>STNLVAEPFAKLEQDFGGSIGVYAMDTGSGATVSYRAEERFPLCSSFKGFLAAAVLARSQQQAGLLDTPIRYGKNALVPWSPISEKYLTTGMTVAELSAAAVQYSDNAAANLLLKELGGPAGLTAFMRSIGDTTFRLDRWELELNSAIPGDARDTSSPRAVTESLQKLTLGSALAAPQRQQFVDWLKGNTTGNHRIRAAVPADWAVGDKTGTCGVYGTANDYAVVWPTGRAPIVLAVYTRAPNKDDKHSEAVIAAAARLALEGLG[4x]

A major mechanism of carbapenem resistance involves production of carbapenemases, i.e. evolved β-lactamases that inactivate carbapenem antibiotics, which can be divided into two categories: serine-carbapenemases (e.g. Ambler class A KPC-2 and class D OXA-48 types) and metallo-carbapenemases (e.g. NDM and VIM types). With the aim of helping enable agents to overcome carbapenem resistance in Gram-negative pathogens, we analysed carbapenem-substrate derived complexes and identified benzoxaboroles with a C3 acrylic acid group as potential inhibitors. Crystallographic analyses validate the proposed mechanism of binding to carbapenemases, i.e. in a manner relating to their antibiotic substrates.

To investigate the structural basis of inhibition by the chiral benzoxaboroles, we obtained KPC-2:(S)-4a and OXA-48:(R)-4a complex structures by co-crystallisation (ESI†). The KPC-2: (S)-4a structure reveals a covalent bond between boron and Ser70, with hydrogen bonds between the inhibitor and β3 Thr237, α8 Ser130, β3 Thr235, and β3 Thr237 (ESI†). Crystallographic analyses revealed that active site of (S)-4a to KPC-2 and of (R)-4a to OXA-48 involves reaction with the nucleophilic serine. The results show both enantiomers of some of the chiral benzoxaborole derivatives manifest moderate, or potent, inhibition of the carbapenemase KPC-2, demonstrating their potential for inhibition of clinically relevant SBLs. In all cases, the (S)-configured compounds (4a, 4c, 4f, 4j, 4q) were more potent than the corresponding (R)-enantiomers, illustrating how chirality can confer selectivity in boron based SBL inhibitors. The KPC-2 stereoselectivity for the benzoxaborole derivatives is interesting since the penicillin substrates of some of the β-lactamases have a (2S) C-3 carbon adjacent to their C-2 carboxylate. The difference in results for the (R)- and (S)-benzoxaboroles may reflect different distances between their carboxylate and electrophilic boron; the analogous carboxylate to β-lactam distance is proposed to be important with respect to antibacterial activity. Addition of 4a, 4c or 4q at 100 μM substantially reduced the MEM MICs, i.e. by 16-128 fold for the KPC-2 producing E. coli strains; notably, the presence of 10 μM (R)-4a and (S)-4a decreased the MEM MICs to below 2 μg ml−1 for E. coli BAA-2340 and E. coli 11119. Based on these structures and computational results, it is proposed that the C-6 4-methoxyphenoxyl group of (S)-4q, which occupies a hydrophobic subpocket adjacent to OXA-48 active site, forms an additional hydrogen bond with Asn170 of KPC-2 (ESI†). This putative interaction may explain why 4q is more potent than 4a and suggests that further optimization of substituents particularly at C-6 should improve the potency of the series for carbapenemase inhibition.>[2x]MAIVKATDQSFSAETSEGVVLADFWAPWCGPSKMIAPVLEELDQEMGDKLKIVKID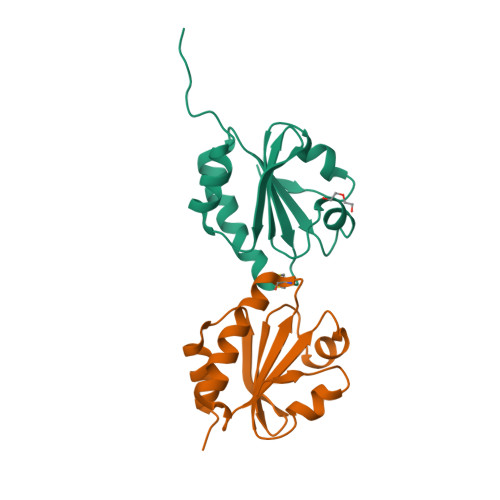VDENQETAGKYGVMSIPTLLVLKDGEVVETSVGFKPKEALQELVNKHLLEHHHHHH> MIEAILFDVDGTLAETEELHRRAFNETF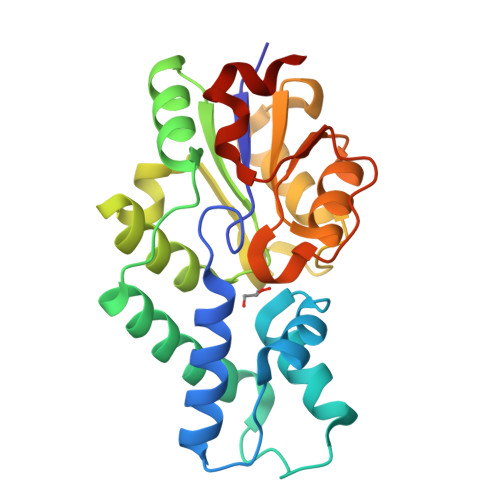AALGVDWFWDREEYRELLTTTGGKERIARFLRHQKGDPAPLPIADIHRAKTERFVALMAEGEIALRPGIADLIAEAKRAGIRLAVATTTSLPNVEALCRACFGHPAREIFDVIAAGDMVAEKKPSPDIYRLALRELDVPPERAVALEDSLNGLRAAKGAGLRCIVSPGFYTRHEEFAGADRLLDSFAELGGLAGLDLTAPVA> GPLGSEWSSSQPATGEKKECWSWESYLEEQKAITAPVSLFQDSQAVTHNKNGFKLGMKLEGIDPQHPSMYFILTVAEVCGYRLRLHFDGYSECHDFWVNANSPDIHPAGWFEKTGHKLQPPKGYKEEEFSWSQYLRSTRAQAAPKHLFVSQSHSPPPLGFQVGMKLEAVDRMNPSLVCVASVTDVVDSRFLVHFDNWDDTYDYWCDPSSPYIHPVGWCQKQGKPLTPPQDYPDPDNFCWEKYLEETGASAVPTWAFKVRPPHSFLVNMKLEAVDRRNPALIRVASVEDVEDHRIKIHFDGWSHGYDFWIDADHPDIHP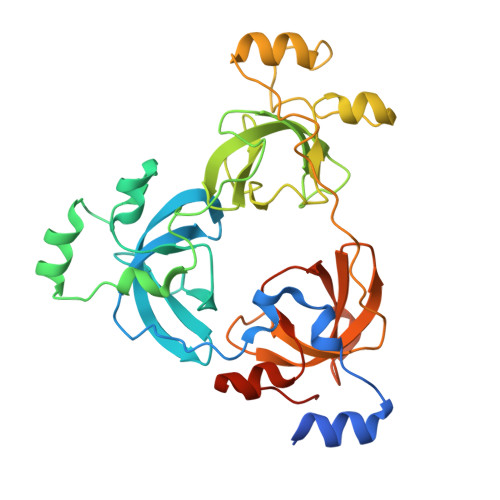AGWCSKTGHPLQPPLGPREPSSASPGG>[6x]MKFYTISSKYIEYLKEFDDKVPNSE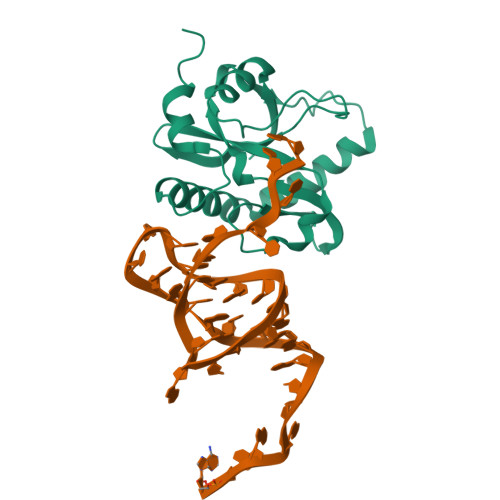DPTYQNPKAFIGIVLEIQGHKYLAPLTSPKKWHNNVKESSLSCFKLHENGVPENQLGLINLKFMIPIIEAEVSLLDLGNMPNTPYKRMLYKQLQFIRANSDKIASKSDTLRNLVLQGKMQGTCNFSLLEEKYRDFGKEAEDTEEGE(5E)-7-{(1R,4S,5S,6R)-5-[(1E,3S)-3-hydroxyoct-1-en-1-yl]-2-oxabicyclo[2.2.1]hept-6-yl}hept-5-enoic acid | C21 H34 O4 | 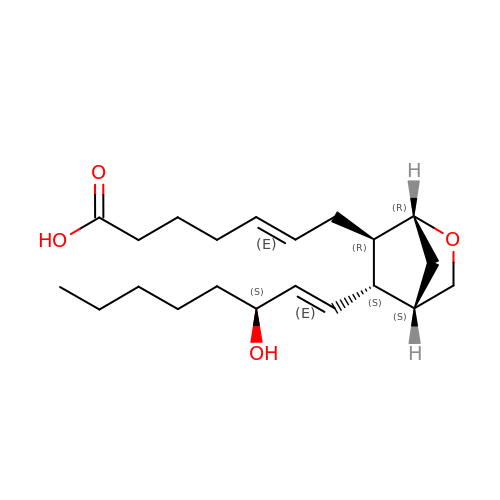DJKDIKIDYDXHDD-JVCJGEKZSA-N> GCGCGCG;> 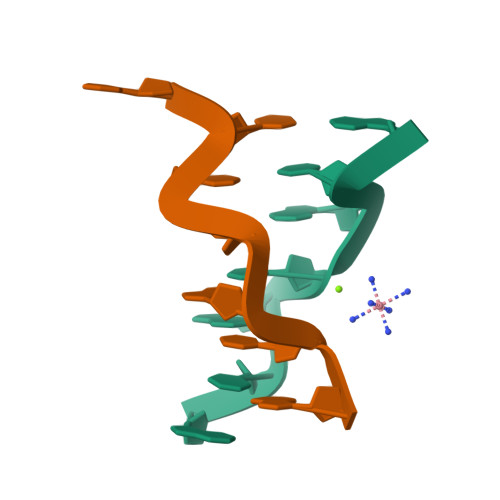CCGCGCG>[2x]GANAYLNLYKIDIPKKIKRLYFYNPDMEPKLFARNLSRVNNFKFQDSNDLVWIEIPDIDFQITPKNVFQYKVEKEEIIKEE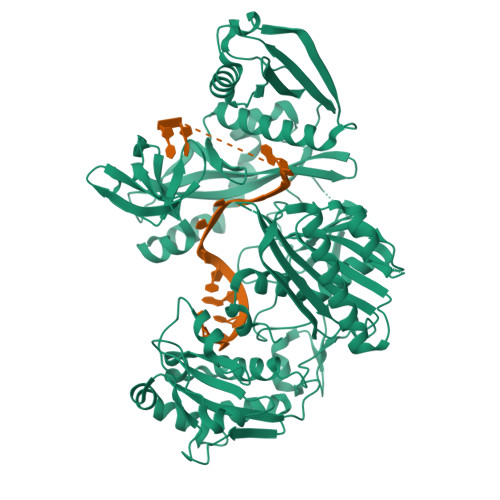EDKKLFVKTLYKYIKKLFLDNDFYFKKGNNFISNSEVFSLDSNENVNAHLTYKIKIHNISNEYYLSILPKFTFLSKEPALESAIKSGYLYNIKSGKSFPYISGLDGILKIDIGNNQIVEVAYPENYLFNFTTRDAEKYGFSKEVHEIYKNKVFEGFKKIPKTLGFLNKITNLNENYQLKDGYKIFINVIYKFKNGESRYAKDVFKYSFYKNEQPLKAIFFFSSKKQFFEVQKSLKELFHNKHSVFYRAAAELGFSKVEFLRDSKTKSSAFLYNPEEFTVKNTEFINQIEDNVMAIVLLDKYIGNIDPLVRNFPDNLILQPILKEKLEDIKPFIIKSYVYKMGNFIPECKPFILKKMEDKEKNLYIGIDLSHDTYARKTNLCIAAVDNTGDILYIGKHKNLELNEKMNLDILEKEYIKAFEKYIEKFNVSPENVFILRDGRFIEDIEIIKNFISYNDTKYTLVEVNKNTNINSYDDLKEWIIKLDENTYIYYPKTFLNQKGVEVKILENNTDYTIEEIIEQIYLLTRVAHSTPYTNYKLPYPLHIANKVALTDYEWKLYIPY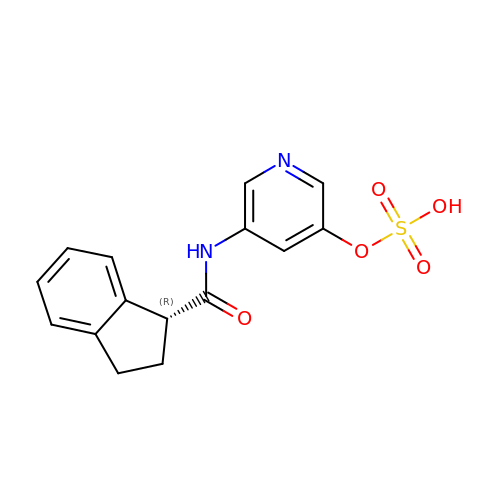(1R)-N-{5-[(dihydroxy-lambda~4~-sulfanyl)oxy]pyridin-3-yl}-2,3-dihydro-1H-indene-1-carboxamide | C15 H14 N2 O5 S | UUXBXVVEARPXOI-CQSZACIVSA-N> YGPDGDPGDPGDPG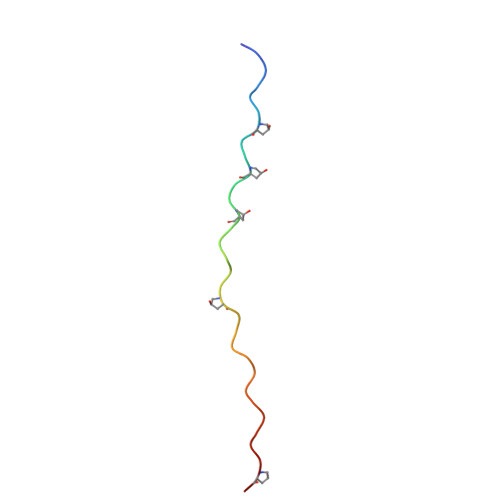PDGKPGPDGPDGPDGDPG>[4x]MKKIGIIGGGQ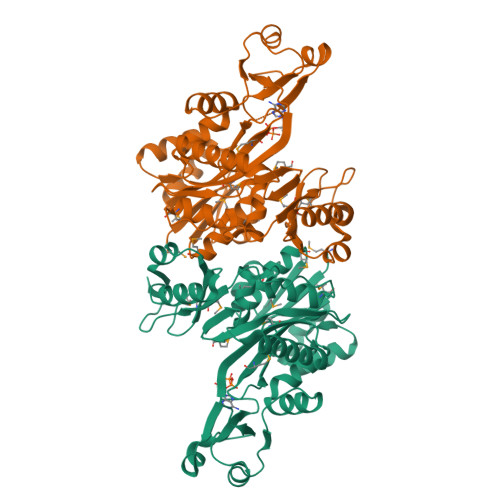LGKMMTLEAKKMGFYVIVLDPTPRSPAGQVADEQIVAGFFDSERIEDLVKGSDVTTYDLEHIDVQTLKKLYNEGYKIHPSPYTLEIIQDKFVQKEFLKKNGIPVPEYKLVKDLESDVREFGFPVVQKARKGGYDGRGVFIIKNEKDLENAIKGETYLEEFVEIEKELAVMVARNEKGEIACYPVVEMYFDEDANICDTVIAPARIEEKYSKIAREIATSVVEALEGVGIFGIEMFLTKQGEILVNEIAPRPHNSGHYTIEACVTSQFEQHIRAIMNLPLGSTELLIPAVMVNLLGEEGYYGKPALIGLEEALAIEGLSLHFYGKKETRPYRKMGHFTVVDRDVERALEKALRAKKILKVVSEEGAMCQG>MKNPLTLSKEEEVLQNLQSFSAHFKQVLKNEKPLVYYGVLKAKAPNWALWVYEKPLKKEIYMNDKEVVVYEPNLFQATITPLKDKTDFFTILKQLKKQTDGSFKTTINKTTYRLVFKDGKPFSLEFKDDMNNLVTITFSQAEINPKIPNEIFVFNPKDENIDIVRQ[2x]

In Gram-negative bacteria, the localization of lipoprotein (Lol) system facilitates the transport of these proteins from the inner membrane to the outer membrane. In Helicobacter pylori, an ε-proteobacterium, lipoprotein transport differs significantly from the canonical and well-studied system in Escherichia coli, particularly due to the absence of LolB and the use of a LolF homodimer instead of the LolCE heterodimer. This study presents the crystal structure of the H. pylori lipoprotein chaperone LolA (LolA-HP) and its interaction with lipopeptide antibiotics such as polymyxin B and colistin. Specifically, H. pylori lacks the LolB receptor protein at the OM and, instead of the LolCE dimer at the IM utilizes a homodimeric LolF, which combines the functions of LolC and LolE.

After X-ray diffraction data were collected, the structure of LolA-HP was determined with molecular replacement using a search model obtained from AlphaFold. The structure was refined to 2.05 Å with final Rwork and Rfree values of 20.2 and 25.2%, respectively. Similar to other LolA structures, LolA-HP comprises a curved antiparallel β-sheet that consists of 12 strands. The last strand, β12, links to β11 through an elongated segment that extends along the outwardly curved surface of the β-sheet. The concave side of the sheet forms a hydrophobic cleft, shielded from the adjacent solvent by the presence of a helix (α2) and an extended loop region between β6 and α2. The base of this cleft is formed by the N-terminal helix, α1. In LolA-EC and other studied LolA structures, there is an additional helix that protects the cleft, which is equivalent to the extended β6α3 loop in LolA-HP. In LolA-HP there is a proline (P99) at the end of β6 that precedes the extended region, but no other prolines are present in the segment that fills the cleft. In LolA-HP, this motif is replaced by an Ala-Pro motif (Ala62, Pro63), and the space that would be occupied by the arginine side chain in LolA-EC is instead filled by a phenylalanine side chain (Phe107) on the α3-helix. Structural comparisons showed that LolA-HP has a deeper hydrophobic cleft but lacks the negative electrostatic potential critical for binding polymyxins.> VTNEKGQAYTEMLQLFNLLQQWNDFYTAENANNLLVACQQLLINYNEPVIKFIN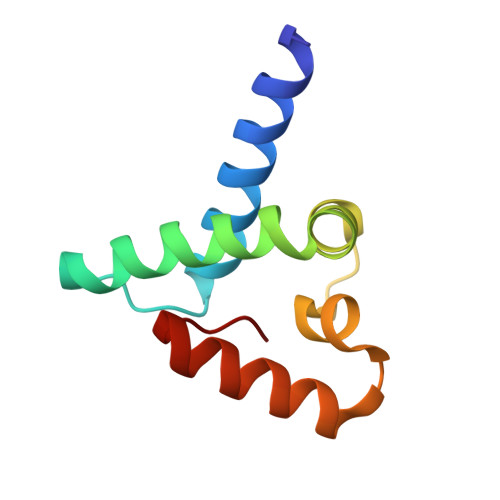DENEDKSLLQYLAGDDGLAQWQFYKGFYNNYNVHIF4-oxidanylidene-4-(6-oxidanylidene-1~{H}-pyridin-3-yl)butanoic acid | C9 H9 N O4 | 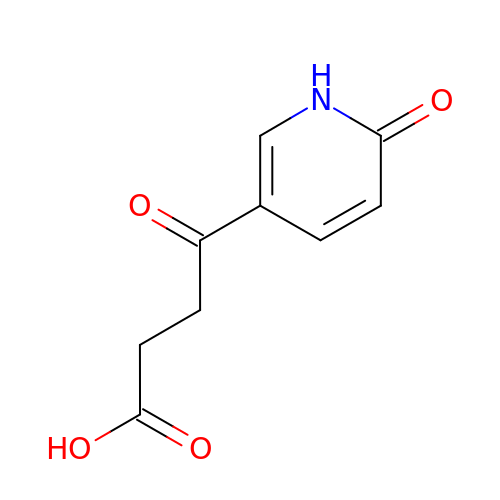OMAJIMAYOJBLJF-UHFFFAOYSA-N> MGSSHHHHHH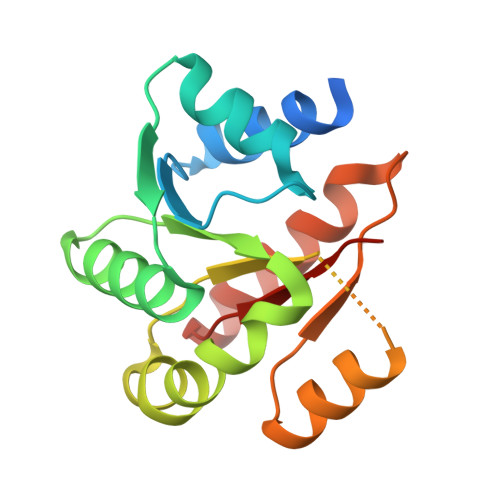SQDPMNSTAERMLSTLTENNYTHFTGVPCSLLKGFFRLLESKEAIEKQNITFIPSIREDSALGVASGMYLGGRKCVMLMQNSGLGYCLNVLTSFNFIYDIPILLLISWRGAYGNDAVEHDIIGEKLTDLLDSVDIPYKELDYENSEGTILDALFLIEKTNRPVAILIKDEI>MLCEIECRALSTAHTRLIHDFEPRDALTYLEGKNIFTEDHSELISKMSTRLERIANFLRIYRRQASELGPLIDFFNYNNQSHLADFLEDYIDFAINEPDLLRPVVIAPQFSRQMLDRKLLLGNVPKQMTCYIREYHVDRVIKKLDEMCDLDSFFLFLHGRAGSGKSVIASQALSKSDQLIGINYDSIVWLKDSGTAPKSTFDLFTDILLMLKSEDDLLNFPSVEHVTSVVLKRMICNALIDRPNTLFVFDDVVQEETIRWAQELRLRCLVTTRDVEISNAA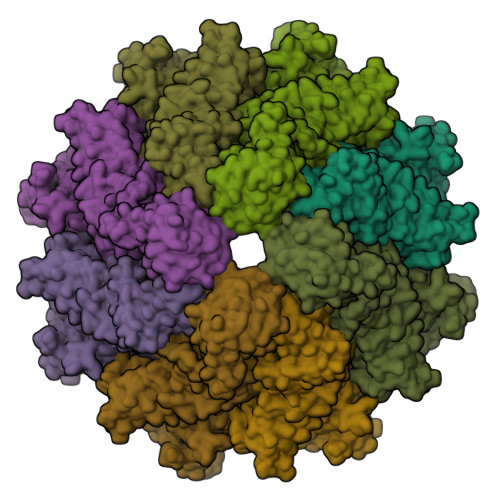SQTCEFIEVTSLEIDECYDFLEAYGMPMPVGEKEEDVLNKTIELSSGNPATLMMFFKSCEPKTFEKMAQLNNKLESRGLVGVECITPYSYKSLAMALQRCVEVLSDEDRSALAFAVVMPPGVDIPVKLWSCVIPVDICSNEEEQLDDEVADRLKRLSKRGALLSGKRMPVLTFKIDHIIHMFLKHVVDAQTIANGISILEQRLLEIGNNNVSVPERHIPSHFQKFRRSSASEMYPKTTEETVIRPEDFPKFMQLHQKFYDSLKNFACC[2x];>[2x]PLFNFLCG> GAAAAACACTGCCTGAATACCGCA;> GCGGTATTCACCACGAT;> TCTTTTGAGTCAGTGGCAGTGTTTT;>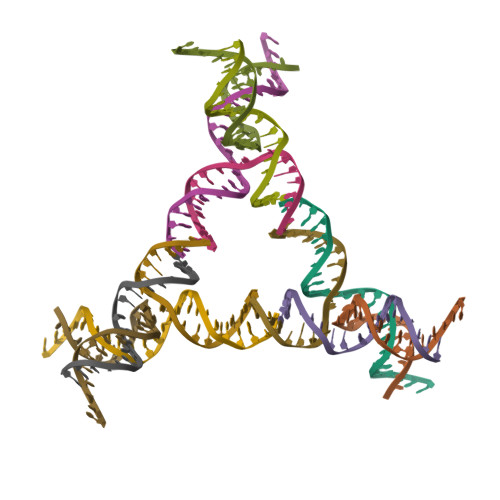 TCGTGGACTGACTCAAAA>MNSTPKGTIYLTFDDGPVNASVEVIKVLNQGGVKATFYFNAWHLDGIGDENEDRALEALKLALDSGHIVGNHSYDHMIHNCVEEFGPTSGADCNATGNHQIHSYQDPVRDAASFEQNLITLEKYLPTIRSYPNYKGYELARLPYTNGWRVTKHFQADGLCATSDNLKPWEPGYVCDPANPSNSVKASIQVQNILANQGYQTHGWDVDWAPENWGIPMPANSLTEAVPFLAYVDKALNSCSPTTIEPINSKTQEFPCGTPLHADKVIVLTHDFLFEDGKRGMGATQNLPKLAEFIRIAKEAGYVFDTMDNYTPRWSVGKTYQAGEYVLYQGVVYKAVISHTAQQDWAPSSTSSLWTNADPATNWTLNVSYEQGDIVNYKGKRYLVSVPHVSQQDWTPDTQNT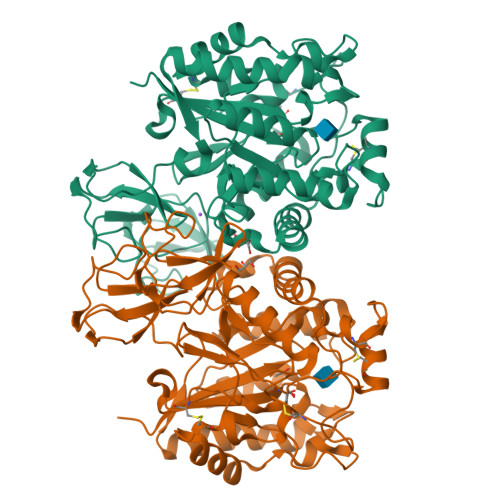LFTALELRRQWSHPQFEK[2x]>MERPAILPSGQILSNIEVHSHRALFDIFKRFRSDDNNLYGAEFDALLGTYCSTLSLVRFLELGLSVACVCTKFPELSYVAEGTIQFEVQQPMIARDGPHPADQPVHNYMIKRLDRRSLNAAFSIAVEALGLISGENLDGTHISSAMRLRAIQQLARNVQAVLDSFERGTADQMLRVLMEKAPPLSLLAPFTLYEGRLADRVACAALVSELKRRVRDDTFFLTKHERNKDAVLDRLSDLVNCTAPSVAVARMTHADTQGRPVDGVLVTTAGVRQRLLHHVLTLADTHADVPVTYGEMVIANTNLVTALVMGKAVSNMDDVARYLLGGEPAPDDGKPVGSARVRADLVVVGDRLVFLEALEKRVYQATQVPYPLVGNLDVTFVMPLGVFKPAADRYARHAGSFAPTPGLPDPRTHPPRAVHFFNKDGVPCHVTFEHAMGTLCHPSFLDVDATLAALRQEPAEVQCAFGAYVADARPDALVGLMQRFLEEWPGMMPVRPRWAAPAAADQLLAPGNADLRLELHPAFDFFVAPEVDVPGPFAVPQVMGQVRAMPRIINGNIPLALCPVDFRDARGFELSVDRHRLAPATVAAVRGAFRDANYPMVFYIIEAVIHGSERTFCALARLVAQCIQSYWRNTHNAAFVNNFYMVMYINTYLGNGELPEDCAAVYKDLLEHVHALRRLIGEFTLPGDPLGNQPQEELNHALADATLLPPLIWDCDPILYRDGLAERLPELRVNGAHFQHILWVEMAQVNFRNVGGGLVHNRPVRNENQPLHPHHDAEWSVLSKIYYYAVVPAFSRGNCCTMGVRYDRVYQLVQTMVVPETDEEVGTDDPRHPLHPRNLVPNSLNVLFHNACVAVDADAMLILQETVTNMAERTTPLLASVAPDAGMATVATRDMRTHDGSLHHGLLMMAYQPNDATLLEGAFFYPAPVNALFACADHLGAMRDVGAEVRAAAQHVPCVPHFLGANYYATVRQPVAQHAAQSRADENTLSYALMAGYFKMSPVAFTHQLRRQLHPGFALTVVRQDRFATENVLFAEKASESYFMGQMQVARTESGGGLHLQLTQPRANVDLGVGFTAAYAAAALRAPVTDMGNLPQNLFATRGAPPMLDADADDYLRRTVNAGNRLAPVPVFGQMLPQVPAGLARGQQSVCEFIATPVSVDLAYFRRACNPRGRAAGEVHGEEGLMFDHSHADPAHPHRATANPWASQRHSYADRLYNGQYNMSGPAYSPCFKFFTPAEAVAKSRGLARLIADTGAAASPTSNGEYQFKRPVGAGELVEDPCALFQEAYPPLCASDSALLRTPLGAEEHFAQYLIRDESPLKGCFQHASA[16x];>[10x]MEVDIALPTLSPGDLSALQRCEGRVVFLETLRRHATLREVALPCGGDVLAAMAAYRRRFAAVITRVTPHRMLATPLGVGGRGQSLVLQNTGPFDLTNGDHVCLVPPLLGDECLRLTSANLELRFPMTLPLAQARELTARVVARAAETLRGGAPARGADVVFSNGRRYQLPPPHRDNAEAATRSLVLNMIFLLNEGAVILLSLIPNLLTLGAQDGYANAVIQLGSATRELGQLVRQPPPPLPQDHARRFCVFEALEAWIASASRLGDTLGTRPVARVCIFDGPPTVPPGEKAAVVEV;>[10x]MSVQIGNGLLMVVAPGTLTVGSARARLIRQVTLADFCEPQAERPGLVVLALRHPADLAGAAYAATPPGKNHRDLEEAWLALDEGGRGLGGDGIRASVVSLNFLVAAAENADDALRAHVTTNYRDRRTAARLERFATVLRAMIRSHVFPHRALHVLGGLLGHVTQDRLASVTCVARGDQEAARTNDMAARRSQVHVPACALMDVDRELRLGGDDGLRFAYLVFVYTQRHRREALRVHVAVSRLPELGDALSFLLAGTRVDNAIHGTDEADAPAAPAAAAAFPAYLFNDPRSARCPTGRLNTPAAEALPVWAPDMRGRATRNSCMYAAYVRLGTVERVVRRAERCGSVDLPLAHMERFTWDVGAWEECFF;>MSFDPNNPRTITAQTLEGALPVDILLRLNRATGLQMDAAEAHAIVEDARRTLFIGTSLALVNLRRAHDKHLVERQPMFATSDYSSWARPTVGLKRTFCPRPPP[15x]

The PRV capsid, similar to other herpesviruses, has a triangulation (T) number of 16 and is composed of major capsid proteins (MCPs), small capsid proteins (SCPs), and triplexes. The MCP (VP5) is encoded by UL19 and forms pentamer (penton) and hexamer (hexon) in the capsid. The hexon MCP is decorated with the SCP (VP26 protein, encoded by UL35), whereas the penton MCP lacks decoration. The triplexes, each composed of one VP19C protein (Tri1, encoded by UL38) and two VP23 proteins (Tri2, encoded by UL18), anchor to the capsid floor via Tri1 N-anchor.

The A-capsid is empty, whereas the C-capsid is fully packed with genomic DNA, and the B-capsid contains a core of scaffold proteins but without genomic DNA. It has been speculated that A- and B-capsids assemble with abortive genomic DNA packing. Here, we use cryo-EM to image both the PRV empty capsid resulted from abortive DNA packing (A-capsid) and mature capsids fully packed with DNA (C-capsid). From the same dataset, we selected a total of 14,252 and 8899 particles for PRV C-capsid and A-capsid, respectively, and, by imposing icosahedral symmetry, obtained three-dimensional (3D) reconstructions at resolutions of 4.43 and 4.53 Å, respectively. Local reconstructions were then carried out to finally obtain the cryo-EM structures of the C-capsid 5-, 3-, and 2-fold sub-regions at 3.31, 3.46, and 3.43 Å, respectively, and the A-capsid 5-, 3-, and 2-fold sub-regions at 3.64, 3.50, and 3.41 Å, respectively. The structures of the PRV A-capsid and C-capsid are nearly identical except for the presence of CATCs in the latter. Because the Tf triplex is located at the icosahedral 3-fold axis, the densities were smeared during 3D reconstruction with imposed icosahedral symmetry. The models of the asymmetric units derived from icosahedral reconstructions of the A- and C-capsids are nearly identical, with a root mean square deviation of 0.298 Å over 26,091 atoms, with the Cα positions of the two models aligned. In contrast, our structural information confirmed that CATC binding or not does not affect Ta orientation at the penton vertex, as the orientations of Ta from A-capsid (CATC absent) or C-capsid (CATC present) are the same. However, the same strategy was unable to procure a 3D reconstruction of the portal vertex of the PRV A-capsid, possibly indicating the instability or altered structural dynamics of the portal vertex in the A-capsid.>[60x]MPWWYRRRSYNPWRRRNWFRRPRKTIYRRYRRRRRWVRRKPFYKRKIKRLNIVEWQPKSIRKCRIKGMLCLFQTTEDRLSYNFDMYEESIIPEKLPGGGGFSIKNISLYALYQEHIHAHNIFTHTNTDRPLARYTGCSLKFYQSKDIDYVVTYSTSLPLRSSMGMYNSMQPSIHLMQQNKLIVPSKQTQKRRKPYIKKHISPPTQMKSQWYFQHNIANIPLLMIRTTALTLDNYYIGSRQLSTNVTIHTLNTTYIQNRDWGDRNKTYYCQTLGTQRYFLYGTHSTAQNINDIKLQELIPLTNTQDYVQGFDWTEKDKHNITTYKEFLTKGAGNPFHAEWITAQNPVIHTANSPTQIEQIYTASTTTFQNKKLTDLPTPGYIFITPTVSLRYNPYKDLAERNKCYFVRSKINAHGWDPEQHQELINSDLPQWLLLFGYPDYIKRTQNFALVDTNYILVDHCPYTNPEKTPFIPLSTSFIEGRSPYSPSDTHEPDEEDQNRWYPCYQYQQESINSICLSGPGTPKIPKGITAEAKVKYSFNFKWGGDLPPMSTITNPTDQPTYVVPNNFNETTSLQNPTTRPEHFLYSFDERRGQLTEKATKRLLKDWETKETSLLSTEYRFAEPTQTQAPQEDPSSEEEEESNLFERLLRQRTKQLQLKRRIIQTLKDLQKLE

Anelloviruses are nonpathogenic viruses that comprise a major portion of the human virome. Our determination of the LY1 structure demonstrates that ORF1 encodes the capsid protein and that anelloviruses evolved a novel spike domain that extends around the 5-fold axis to form a crown structure. The particle, formed by 60 jelly roll domain-containing ANV capsid proteins, forms an icosahedral particle core from which spike domains extend to form a salient part of the particle surface. The base of the spike domain, the P1 subdomain, shares some sequence conservation between ANV strains while a hypervariable region, forming the P2 subdomain, is at the spike domain apex.

Our initial efforts to study the structure of an ANV particle, derived from a Betatorquevirus isolate called LY1, were performed with the full-length ORF1 (residues 1–672) expressed in insect cells (Sf9) using a baculovirus system (pFastbac, Thermo Fischer) encoding a codon-optimized ORF1 construct. However, full-length ORF1 particles lacked the structural homogeneity and symmetry expected of viral particles. Initial expression of the ORF1 protein in insect cells (Sf9) suggested a proteolytically susceptible region of ORF1 that resulted in the removal of the C-terminus. To prevent potential proteolysis from occurring in the ARM by trypsin-like proteases, we designed the LY1 ΔARM construct wherein residues 2–45 are deleted. However, we continued to observe a smaller ORF1 band accumulating below the 62 kDa marker during purification, confirming the proteolysis was not limited to the ARM region. To identify the region of proteolysis, we generated polyclonal antibodies to peptides from the jelly roll domain at the extreme N-terminus (residues 46–58) and the C-terminal domain at the C-terminus (residues 635–672) of the LY1 ΔARM construct and confirmed the presence of the N-terminal peptide of the LY1 ΔARM fragment and the absence of the C-terminal peptide by western blot analysis. EM analysis of the LY1 ΔARM fragment showed that the particles formed were more homogeneous and symmetric in morphology relative to the particles formed by full-length ORF1. With the C-terminus of the ORF1 polypeptide removed, the protein spontaneously formed symmetric 60-mer particles, as determined by cryogenic electron microscopy (cryo-EM). We determined the cryo-EM structure of the virus-like particles formed by the insect cell-derived ΔARM fragment to 3.9 Å resolution from 6271 particles and of the mammalian cell-derived LY1 ΔC-Term ORF1 particle using cryo-EM to 2.69 Å resolution from 22,743 particles. Despite being generated in two different cell lines and the presence of the ARM region in the mammalian virus-like particle (which is not visible in the density, suggesting flexibility) the two protomer structures are very similar (1.179 Å root mean square deviation when aligned over residues 48–562).>HHHHHHMAKKVNWYVSCSPRSPEKIQPELKVLANFEGSYWKGVKGYKAQEAFAKELAALPQFLGTTYKKEAAFSTRDRVAPMKTYGFVFVDEEGYLRITEAGKMLANNRRPKDVFLKQLVKWQYPSFQHKGKEYPEEEWSINPLVFVLSLLKKVGGLSKLDIAMFSLTATNNNQVDEIAEEIMQFRNEREKIKGQNKKLEFTENYFFKRF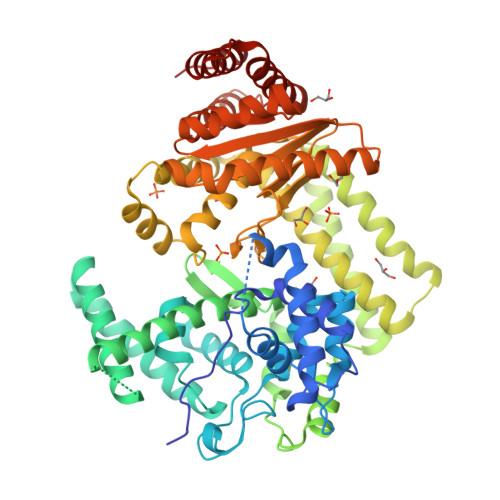EKIYGNVGKIREGKSDSSHKSKIETKMRNARDVADATTRYFRYTGLFVARGNQLVLNPEKSDLIDEIISSSKVVKNYTRVEEFHEYYGNPSLPQFSFETKEQLLDLAHRIRDENTRLAEQLVEHFPNVKVEIQVLEDIYNSLNKKVDVETLKDVIYHAKELQLELKKKKLQADFNDPRQLEEVIDLLEVYHEKKNVIEEKIKARFIANKNTVFEWLTWNGFIILGNALEYKNNFVIDEELQPVTHAAGNQPDMEIIYEDFIVLGEVTTSKGATQFKMESEPVTRHYLNKKKELEKQGVEKELYSLFIAPEINKNTFEEFMKYNIVQNTRIIPLSLKQFNMLLMVQKKLIEKGRRLSSYDIKNLMVSLYRTTIESERKYTQIKAGLEETLNNWVVDKEVRF[2x]>DREKIYQWINELSSPETRENALLELSKKRESVPDLAPMLWHSFGTIAALLQEIVNIYPSINPPTLTAHQSNRVCNALALLQCVASHPETRSAFLAAHIPLFLYPFLHTVSKTRPFEYLRLTSLGVIGALVKTDEQEVINFLLTTEIIPLCLRIMESGSELSKTVATFILQKILLDDTGLAYICQTYERFSHVAMILGKMVLQLSKEPSARLLKHVVRCYLRLSDNPRAREALRQCLPDQLKDTTFAQV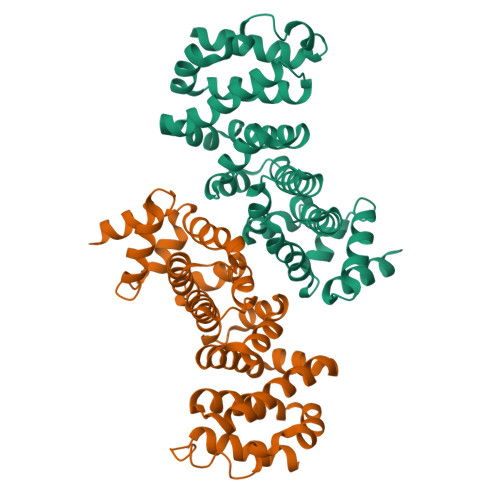LKDDTTTKRWLAQLVKNLQE[4x]>MDVARNGARGSVESPPNRKVYMDYNATTPLEPEVIQAVTEAMKEAWGNPSSSYVAGRKAKDIINTARASLAKMIGGKPQDIIFTSGGTESNNLVIHSTVRCFHEQQTLQGRTVDQISPEEGTRPHFITCTVEHDSIRLPLEHLVEDQVAEVTFVPVSKVNGQVEVEDILAAVRPTTCLVTIMLANNETGVIMPISEISRRIKALNQIRAASGLPRVLVHTDAAQALGKRRVDVEDLGVDFLTIVGHKFYGPRIGALYVRGVGKLTPLYPMLFGGGQERNFRPGTENTPMIAGLGKAADLVSENCETYEAHMRDIRDYLEERLEAEFGKRIHLNSRFPGVERLPNTCNFSIQGSQLRGYMVLAQCQTLLASVGASCHSDHEDRPSPVLLSCGIPVDVARNAVRLSVGRSTTRAEVDLIVQDLKQAVNQLEGPV[2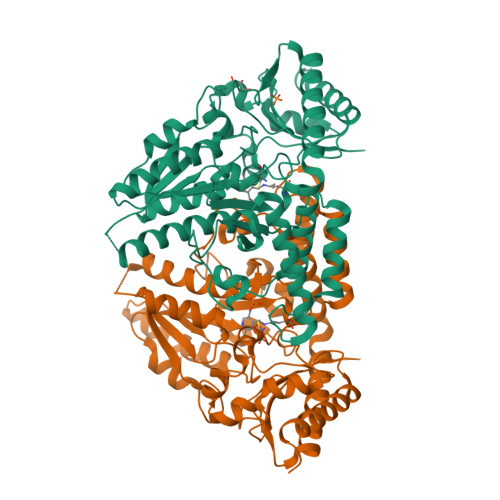x]>MSEEKVVAVIMVGGPTKGTRFRPLSFNTPKPLIPLAGQPMIHHPISACKKISNLAQIFLIGFYEEREFALYVSSISNELKIPVRYLKEDKPHGSAGALYYFRDRIMEEKPSHVFLLNCDVCCSFPLQGILDAHRRYGGIGTMLVIKVSAEAASQFG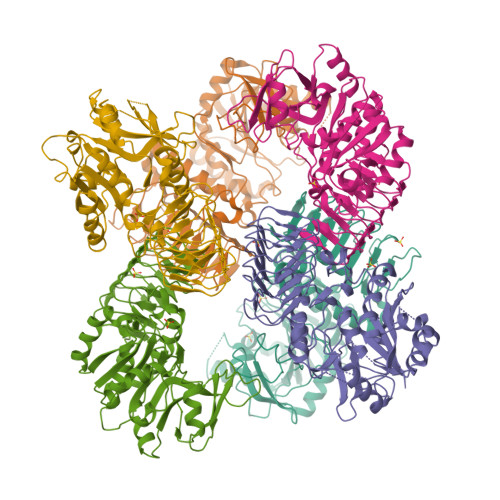ELIADPDTKELLHYTEKPETFVSDLINCGVYVFTSDIFNAIEEVYSQIRDTSSNYQSATRSVPADFVRLDQDILSPLAGKKQLYTYENKDFWEQIKTPGKSLKCSALYLSQFRETSPHILASGDGTNRKPTIIGDVYIHPSVKLHPTAKIGPNVSISANVRVGPGVRLISCIILDDVEIKENAVVINSIIGWKSSIGRWSRVQASGDYNDRLGITILGEAVTVEDEVAVIGSIVLQNKTLNVSVQDDIIL[3x];>MKALILVGGFGTRLRPLTLSFPKPLVDFANKPMILHQIEALKAVGVDEVVLAINYQPEVMLNFLKDFETKLEIKITCSQETEPLGTAGPLALARDKLLDGSGEPFFVLNSDVISEYPLKEMLEFHKSHGGEASIMVTKVDEPSKYGVVVMEESTGRVEKFVEKPKLYVGNKINAGIYLLNPSVLDKIELRPTSIEKETFPKIAAAQGLYAMVLPGFWMDIGQPRDYITGLRLYLDSLRKKSPAKLTSGPHIVGNVLVDETATIGEGCLIGPDVAIGPGCIVESGVRLSRCTVMRGVRIKKHACISSSIIGWHSTVGQWARIENMTILGEDVHVSDEIYSNGGVVLPHKEIKSNILKPEIVM[3x]>DEASGIGPEEHFPEVPEIEPMGPVCPFRCQCHLRVVQCSDLGLEKVPKDLPPDTALLDLQNNKITEIKDGDFKNLKNLHTLILINNKISKISPGAFAPLVKLERLYLSKNQLKELPEKMPKTLQELRVHENEITKVRKSVFNGLNQMIVVELGTNPLKSSGIENGAFQGMKKLSYIRIADTNITTIPQGLPPSLTELHLDGNKITKVDAASLKGLNNLAKLGLSFNSISAVDNGSLANTPHLRELHLNNNKLVKVPGGLADHKYIQVVYLHNNNISAIGSNDFCPPGYNTKKASYSGVSLFSNPVQ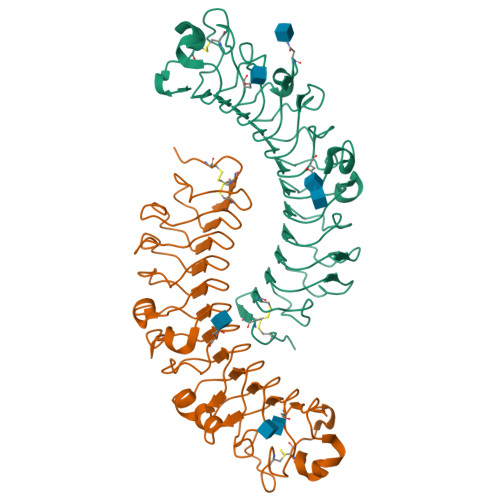YWEIQPSTFRCVYVRAAVQLGNY[2x]> LKESPSGYLRSGEGDTGCGELVWVGEPLTLRTAETITGKYGVWMRDPKPTYPYTQETTWRIDTVGTDVHQVFEYDLISQFMQGY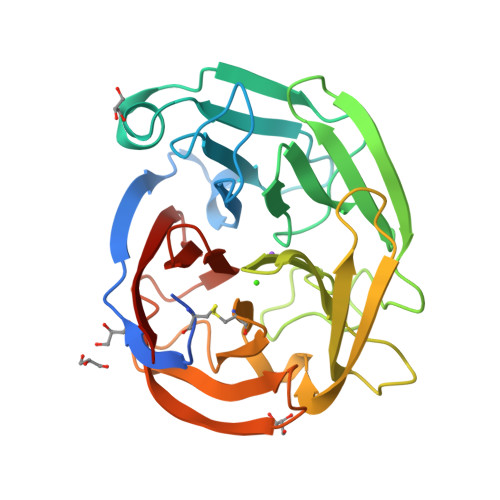PSKVHILPRPLESTGAVVYSGSLYFQGAESRTVIRYELNTETVKAEKEIPGAGYHGQFPYSWGGYTDIDLAVDEAGLWVIYSTDEAKGAIVLSKLNPENLELEQTWETNIRKQSVANAFIICGTLYTVSSYTSADATVNFAYDTGTGISKTLTIPFKNRYKYSSMIDYNPLEKKLFAWDNLNMVTYDIKLSKM> GSHMSRELKTVSADCKKEAIEKCAQWVVRDCRPFSAVSGSGFIDMIKFFIKVGAEYGEHVNVEELLPSPITLSRKVTSDAKEKKALISREIKSAVEKDGASATIDLWTDNYIKR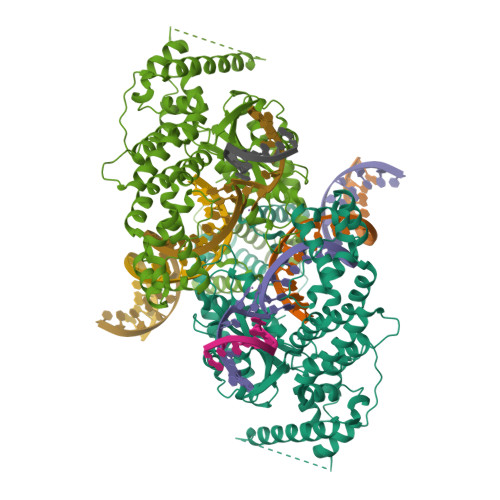NFLGVTLHYHENNELRDLILGLKSLDFERSTAENIYKKLKAIFSQFNVEDLSSIKFVTDRGANVVKSLANNIRINCSSHLLSNVLENSFEETPELNMPILACKNIVKYFKKANLQHRLRSSLKSECPTRWNSTYTMLRSILDNWESVIQILSEAGETQRIVHINKSIIQTMVNILDGFERIFKELQTCSSPSLCFVVPSILKVKEICSPDVGDVADIAKLKVNIIKNVRIIWEENLSIWHYTAFFFYPPALHMQQEKVAQIKEFCLSKMEDLELINRMSSFNELSATQLNQSDSNSHNSIDLTSHSKPVSPSDEFEFYRKEIVILSEDFKVMEWWNLNSKKYPKLSKLALSLLSIPASSAASERTFSLAGNIITEKRNRIGQQTVDSLLFLNSFYKNFCKLDI> TSSATSSSSMILKYPYRVVDTHEKLKEAVTSLQGARSIALDIEAFCTTDQAKQLGRISLVQACSDAKPVVFLFDVLTLTPDVFVKDMQSLLSDREIRKLFFDCRRDVEALSCQLGVKPEGVLDLQVFFTAIQWKLRSVNRRSGMGYVLKSVAGLTRQEGDSAVQTAMTLGNRPVWDIRPLPDHFLEYAAGDVRHILLLSNYLVGNKDVPVDVVAVERLTAQY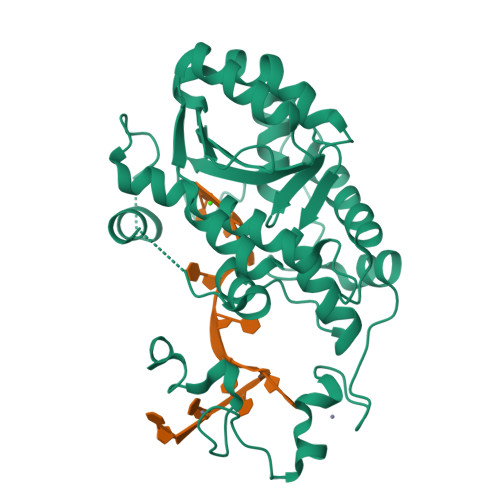VEHYAVGKPVITEADATPAEVNRAWLERYIGPGGGCHFCGAKGHTEAECFKKQNGKAKCSFCGEVGHTARNCFKKHPQLL>MDERDALRISREIAGEVRKAIASMPLRERVKDVGMGKDGTPTKAADRVAEDAALEILRKERVTVVTEESGVLGEGDVFVALDPLDGTFNATQGIPVYSVSLCFSYSDKLKDAFFGYVYNLATGDEYYADSSGAYRNGERIEVSDAEELYCNAIIYYPDRKFPFERMRIFGSAATELCFFADGSFDCFLDIRPGKMLRIYDAAAGVFIAEKAGGKVTELDGESLGNKKFDMQERL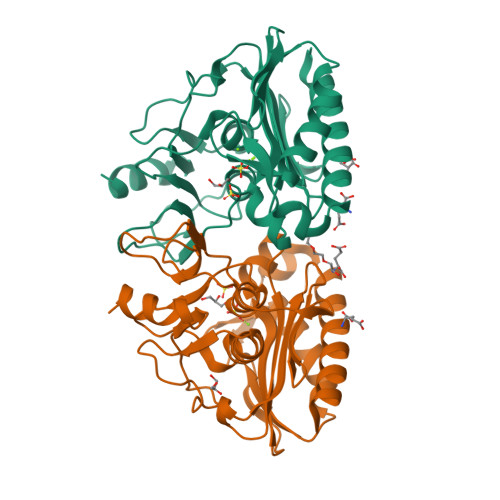NIVAANEKLHPKLLELIK[2x]> HPETLVKVKDAEDQLGARVGYIELDLNSGKILESFRPEERFPMMSTFKVLLCGAVLSRVDAGQEQLGRRIHYSQNDLVEYSPVTEKHLTDGMTVRELCSAAITMSDNTAANL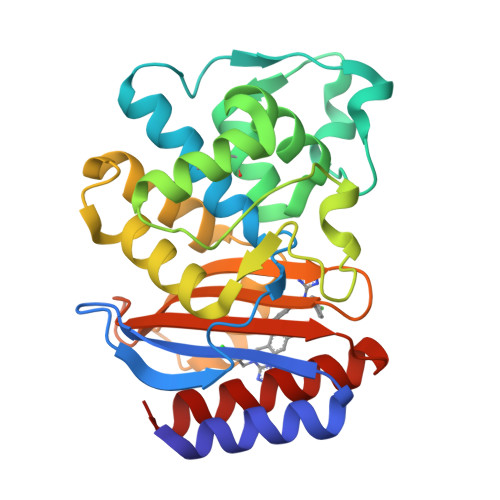LLTTIGGPKELTAFLHNMGDHVTRLDRWEPELNEAIPNDERDTTTPAAMATTLRKLLTGELLTLASRQQLIDWMEADKVAGPLLRSALPAGWFIADKSGAGERGSRGIIAALGPDGKPSRIVVIYTTGSQATMDERNRQIAEIGASLIKHW> AAQTNAPWGLARISSTSPGTSTYYYDESAGQGSCVYVIDTGIEASHPEFEGRAQMVKTYYYSSRDGNGHGTHCAGTVGSRTYGVAKKTQLFGVKVLDDNGSGQYSTIIAGMDFVASDKNNRNCPKGVVASLSLGGGYSSSVNSAAARLQSSGVMVAVAAGNNNADARNYSPASEPSVCTVGASDRYDRRSSFSNYGSVLDIFGPGT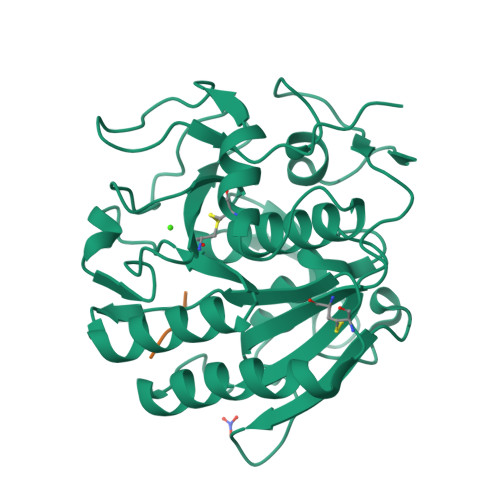DILSTWIGGSTRSISGTSMATPHVAGLAAYLMTLGKTTAASACRYIADTANKGDLSNIPFGTVNLLAYNNYQA;> VLLH>FDHDFAISTSFHGIHNIVQNRSKIRRVLWLVVVLGSVSLVTWQIYIRLLNYFTWPTTTSIEVQYVEKMEFPAVTFCNLNRFQTDAVAKFGVIFFLWHIVSKVLHLQEITANSTGSREATDFAASHQNFSIVEFIRNKGFYLNNSTLLDCEFFGKPCSPKDFAHVFTEYGNCFTFNHGETLQAKRKVSVSGRGLSLLFNVNQEAFTDNPALGFVDAGIIFVIHSPKKVPQFDGLGLLSPVGMHARVTIRQVKTVHQEYPWGECNPNIKLQNFSSYSTSGC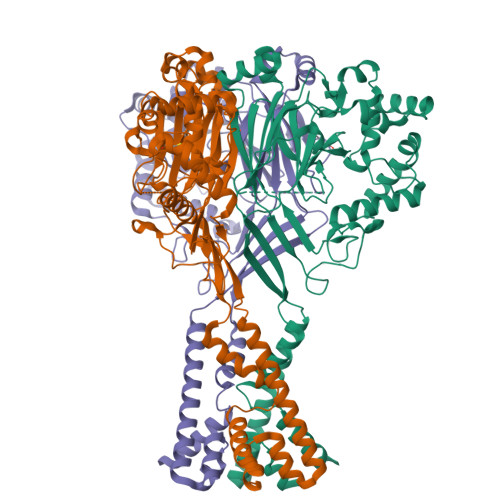LKECKAQHIKKQCGCVPFLLPGYGIECDLQKYFSCVSPVLDHIEFKDLCTVGTHNSSCPVSCEEIEYPATISYSSFPSQKALKYLSKKLNQSRKYIRENLVKIEINYSDLNYKITQQQKAVSVSELLADLGGQLGLFCGASLITIIEIIEYLFTNF[3x]> GNLDIAVYWGQNFDERSLEATCDSGNYAYVIIGFLNTFGGGQTPALDISGHSPSGLEPQIKHCQSKNVKVLLSIGGPAGPYSLDSRSDANDLAVYLFNNFLLPPGHSENNPFGNAVLDGIDFHIEHGGPSQYQLLANILSSFRLKGTEFALTAAPQCVYPDPNLGTVINSATFDAIWVQFYNNPQCSYSSGNAEALMNAWREWSMKARTKKVFLGFPAHPDAAGSGYMPPAKVKFHVFPAAKKSYKFGGIMLWDSYWDTV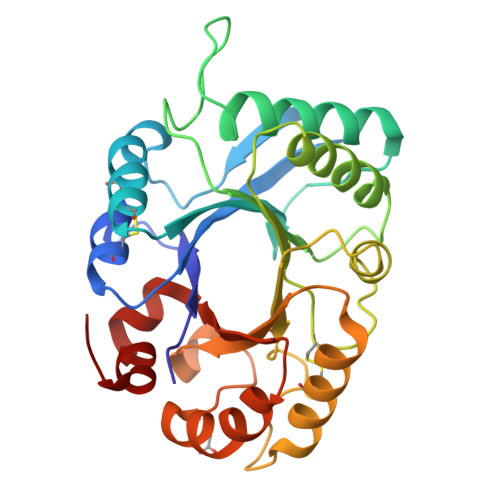SQFSNKILGDGV> GSHLWQMDNTHWNKTIIWVAVETNSGLVEAQVIPEETALQVALCILQLIQRYTVLHLHSDNGPCFTAHRIENLCKYLGITKTTGIPYN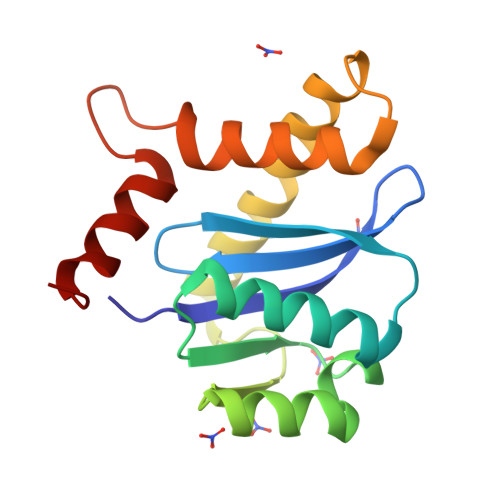PQSQGVVERAHRDLKDRLAAYQGDCETVEAALSLALVSLNKKRGGIGGHTPYEIYLESEHTKYQ5'-deoxy-5'-[(3-{[(4-methylphenyl)carbamoyl]amino}propyl)(propan-2-yl)amino]adenosine 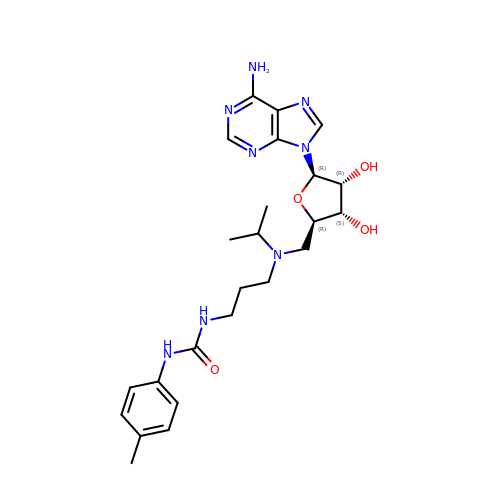| C24 H34 N8 O4 | KQTSVJQPAVOUSL-ZDXOVATRSA-N> MDQKQIEEIVRSVMASMGQAAPAPSEAKCATTNCAAPVTSESCALDLGSAEAKA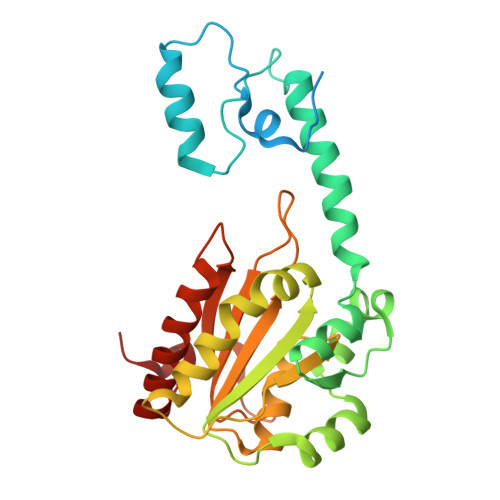WIGVENPHRADVLTELRRSTVARVCTGRAGPRPRTQALLRFLADHSRSKDTVLKEVPEEWVKAQGLLEVRSEISDKNLYLTRPDMGRRLCAEAVEALKAQCVANPDVQVVISDGLSTDAITVNYEEILPPLMAGLKQAGLKVGTPFFVRYGRVKIEDQIGEILGAKVVILLVGERPGLGQSESLSCYAVYSPRMATTVEADRTCISNIHQGGTPPVEAAAVIVDLAKRMLEQKASGINMTR>[2x]MGSSHHHHHHSQDPNSISTTMSSYSIQQSQKMLTQLQIDYATNTSSNTVVAYLHNVGETTISYLQNSVVYFGPN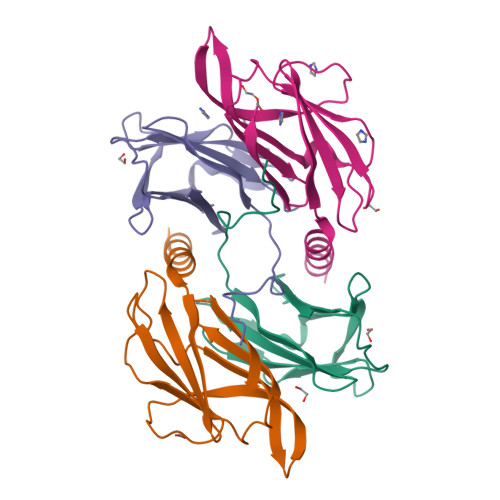GQLQPVGYNSGSSPYWTVTSNSLQPGSVVKIIIYLSSPLSSNQYYTIQIVTPNGYTVSYMF;>MGSSHHHHHHSQDPNSNQAQELNHELELEQLETKITVSSVSLTGSTLNVVLENNGSTNLYDFQGFSVIVQYYANISNISTFNLSLYNYTKNSNPSPYYWTINTPLLAPGSQATLTIILPYPPYPNTQATVVIVTNYGPSVIWRGSL[2x]> MGSSHHHHHHSQDPNSMPDNTIQWDKDADGIVTLTMDDPSGSTNVMNEAYIESMGKAVDRLVAEKDSITGVVVASAKKTFFAGGDVKTMIQARPEDAGDVFNTVETIKRQLRTLETLGKPVVAAINGAALGGGLEIALACHHRIAADVKGSQLGLPEVTLGLLPGGGGVTRTVRMFGIQNAFVSVLAQGTRFKPAKAKEIGLVDELVATVEELVPAAKAWIKEELKANPDGAGVQPWDKKGYKMPGGTPSSPGLAAILPSFPSNLRKQLKGAPMPAPRAILAAAVEGAQVDFDTASRIESRYFASLVTGQVAKNMMQAFFFDLQAINAGGSRPEGIGKTPIKRIGVLGAGMMGAGIAYVSAKAGYEVVLKDVSLEAAAKGKGYSEKLEAKALERGRTTQERSDALLARITPTADAADFKGVDFVIEAVFENQELKHKVFGEIEDIVEPNAILGSNTSTLPITGLATGVKRQEDFIGIAFFSPVDKMPLVEIIKGEKTSDEALARVFDYTLAIGKTPIVVNDSRGFFTSRVIGTFVNEALAML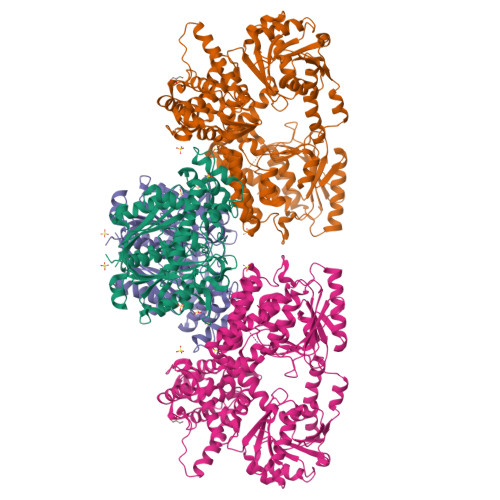GEGVEPASIEQAGSQAGYPAPPLQLSDELNLELMHKIAVATRKGVEDAGGTYQPHPAEAVVEKMIELGRSGRLKGAGFYEYADGKRSGLWPGLRETFKSGSSQPPLQDMIDRMLFAEALETQKCLDEGVLTSTADANIGSIMGIGFPPWTGGSAQFIVGYSGPAGTGKAAFVARARELAAAYGDRFLPPESLLS;> MSEEAFIYEAIRTPRGKQKNGSLHEVKPLSLVVGLIDELRKRHPDLDENLISDVILGCVSPVGDQGGDIARAAVLASGMPVTSGGVQLNRFAASGLEAVNTAAQKVRSGWDDLVLAGGVESMSRVPMGSDGGAMGLDPATNYDVMFVPQSIGADLIATIEGFSREDVDAYALRSQQKAAEAWSGGYFAKSVVPVRDQNGLLILDHDEHMRPDTTKEGLAKLKPAFEGLAALGGFDDVALQKYHWVEKINHVHTGGNSSGIVDGAALVMIGSAAAGKLQGLTPRARIVATATSGADPVIMLTGPTPATRKVLDRAGLTVDDIDLFELNEAFASVVLKFQKDLNIPDEKLNVNGGAIAMGHPLGATGAMILGTMVDELERRNARRALITLCIGGGMGVATIIERV> YWASSQLTQLFLSTDLESLEPTCLSKDTIYQWKVVQTFGDRLRLRQRVLATAIVLLRRYMLKKNEEKGFSLEALVATCIYLSCKVEECPVHIRTICNEANDLWSLKVKLSRSNISEIEFEIISVLDAFLIVHHPYTSLEQAFHDGIINQKQLEFAWSIVNDSYASSLCLMAHPHQLAYAALLISCCNDENTIPKLLDLIKSTDAFKVILCVQRIISIYYFE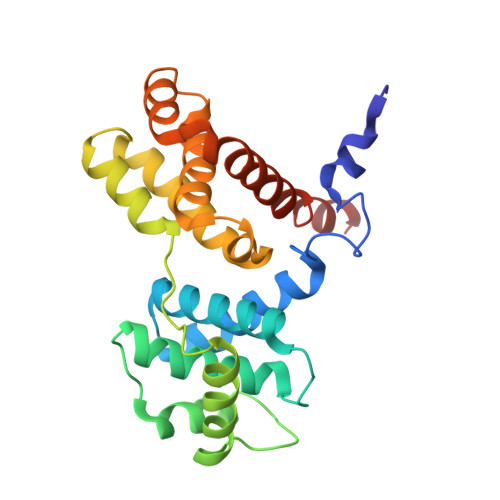DIEAAALEHHHHHH> MKPPSFDYVVADSVEHALRLLADGGDDAKIIAGGQSLVPLLNFRMSRPSLLVDINRVPGLANIRKSDQTIAIGALTRHAKLTTS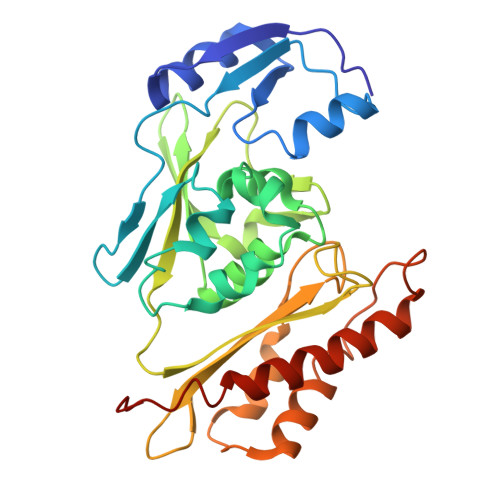KTISQNLPILSEAAAWIAHPQIRNRGTIGGSLAHADAAAELPVVLLALDAYVTAQSLQGERKIPLKELLVSHFVSSILPGELIVEVNVPQLPHGSGAAFDEFSRRHGDYAIGGAASLVTLDEQGKCSRARITVLGGGSTAIRCQEAENILIDSTLSSHDIAAAAHAAVQGLDPVPTVHGSAQYRAQVIRTMVERTLAKALHRARPTKESMDH>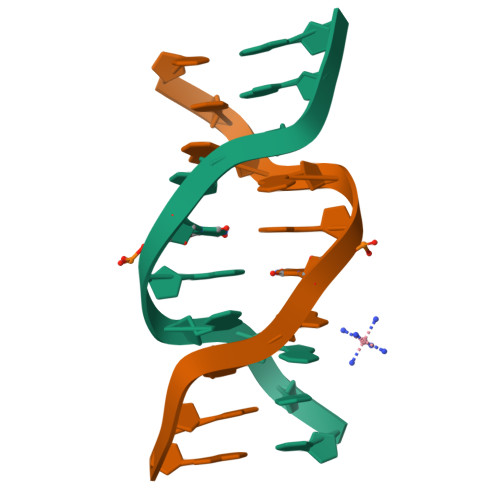[2x]CCGAAUGAGG N5-cyclopropyl-N3-methyl-1-(phenylmethyl)pyrazole-3,5-dicarboxamide | C16 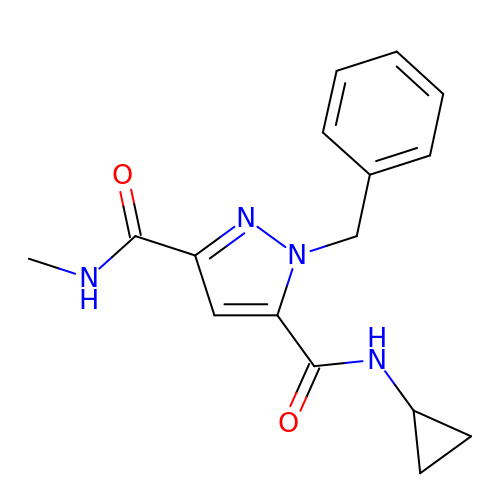H18 N4 O2 | HSYFSGUXNLQCQP-UHFFFAOYSA-N>[6x]MEYVYAALLLHSVGKEINEENLKAVLQAAGV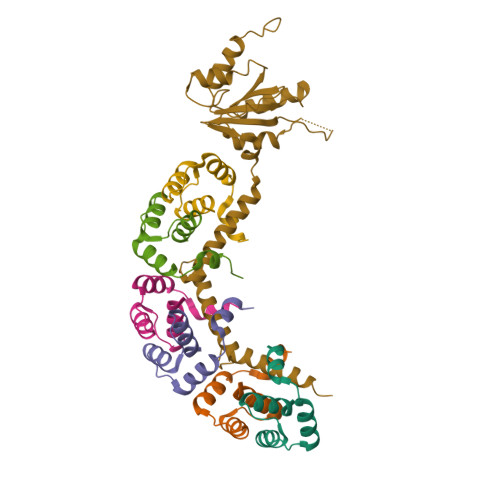EPEEARIKALVAALEGVNIDEVIEKAA;> MAHVAEWKKKEVEELAKLIKSYPVIALVDVSSMPAYPLSQMRRLIRENGGLLRVSRNTLIELAIKKAAKELGKPELEKLVEYIDRGAGILVTNMNPFKLYKFLQQNRQPAPAKPGAVVPKDVVVPAGPTPLAPGPIVGQMQALGIPARIEKGKVTIQKDTTVLKAGEVITPELANILNALGIQPLEVGLDVLAVYEDGIVYTPDVLAIDEQEYIDMLQKAYMHAFNLAVNIAYPTPETIEAIIQKAFLNAKTVAIEAGYITKETIQDIIGRAFRAMLLLAQQLP>[4x]MNHKVHMMSKPVLYYDDISPPVRGVLLTVAALGIKDQVELKLVRLFEREHLLEDFVKLNPLHAVPVLKHDDLVLTDSHAIIMYLC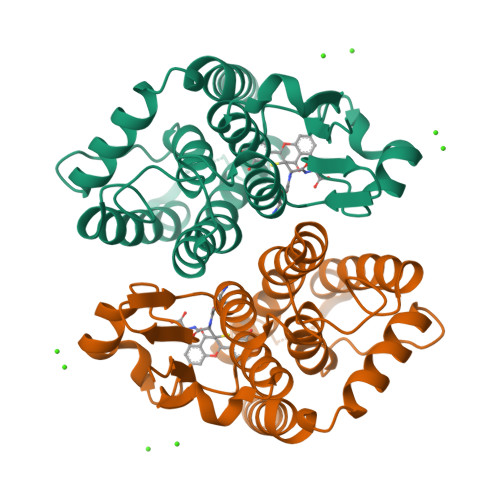DIFGQDGDFSLKDPKQRARVHNRLCFNNAVLFQRESIVMRGLINRSIVTLEDHHLKPVQEAYDCLEVYLTNSKFVACDQLTVADFPIVACMSTVGMVCPLSTSRWPKTAAWFETMKQLPYYQQANQVGVDKLKERLHAVMKK> MEL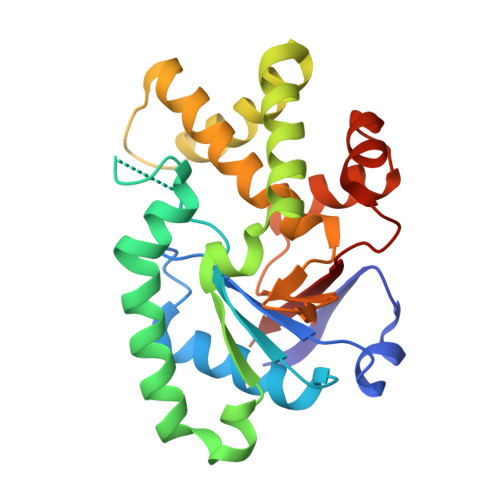HQIRGCHKNDIELKKYNIGVAISLGNKWFSIDNIEKLVKWSLLHTKEYVIIYIADSIHGINLSVRNKLSDSHAEEVAIRYGRNLFIKIKERVSLSFSQDEQAKIIYATWSDIADSKYKEKVKYLYNLYDKNINFKNYIENFVKEWVSKEKRTFNNNEINKFGRYILEQLPELMVQVKARGVLFEAYVYPYKTRITEFVGLLQKGEIFPEIKTNILDNHPKIFLEVRE>[2x]MKTIIINGVQFNTDEDTTILKFARDNNIDISALCFLNNCNNDINKCEICTVEVEGTGLVTACDTLIEDGMIINTNSDAVNEKIKSRISQLLDIHEFKCGPCNRRENCEFLKLVIKYKARASKPFLPKDKTEYVDER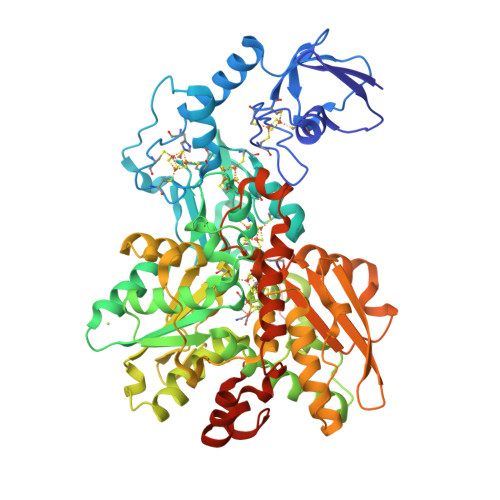SKSLTVDRTKCLLCGRCVNACGKNTETYAMKFLNKNGKTIIGAEDEKCFDDTNCLLCGQCIIACPVAALSEKSHMDRVKNALNAPEKHVIVAMAPSVRASIGELFNMGFGVDVTGKIYTALRQLGFDKIFDINFGADMTIMEEATELVQRIENNGPFPMFTSACPGWVRQAENYYPELLNNLSSAKSPQQIFGTASKTYYPSISGLDPKNVFTVTVMPCTSKKFEADRPQMEKDGLRDIDAVITTRELAKMIKDAKIPFAKLEDSEADPAMGEYSGAGAIFGATGGVMEAALRSAKDFAENAELEDIEYKQVRGLNGIKEAEVEINNNKYNVAVINGASNLFKFMKSGMINEKQYHFIEVMACHGGCVNGGGQPHVNPKDLEKVDIKKVRASVLYNQDEHLSKRKSHENTALVKMYQNYFGKPGEGRAHEILHFKYKKSAWSHPQFEK> MNQTDTSPIRLRRSWNTSEIEALFDEHAGRIDPRIYTDEDLYQLELERVFARSWLLLGHETQIRKPGDYITTYMGEDPVVVVRQKDASIAVFLNQCRHRGMRICRADAGNAKAFTCSYHGWAYDTAGNLVNVPYEAESFACLNKKEWSPLKARVETYKGLIFANWDENAVDLDTYLGEAKFYMDHMLDRTEAGTEAIPGVQKWVIPCNWKFAAEQFCSDMYHAGTTSHLSGILAGLPE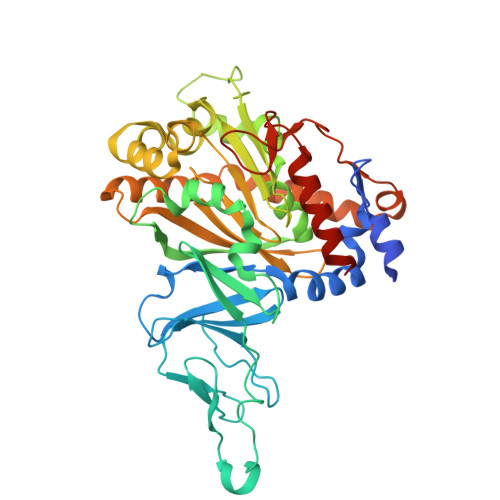DLEMADLAPPTVGKQYRASWGGHGSGFYVGDPNLMLAIMGPKVTSYWTEGPASEKAAERLGSVERGSKLMVEHMTVFPTCSFLPGINTVRTWHPRGPNEVEVWAFTVVDADAPDDIKEEFRRQTLRTFSAGGVFEQDDGENWVEIQHILRGHKARSRPFNAEMSMDQTVDNDPVYPGRISNNVYSEEAARGLYAHWLRMMTSPDWDALKATR>[8x]MHHHHHHTSLIEQPRWASKDSAAGAASTPDEKIVLEFMDALTSNDAAKLIEYFAEDTMYQNMPLPPAYGRDAVEQTLAGFFTVVSVDAVETFHIG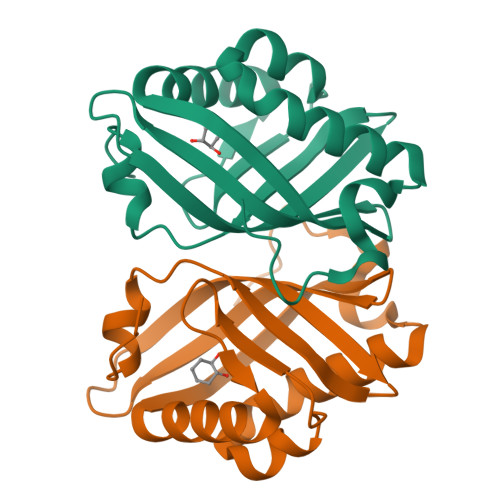SSNGLVYTERVDVLRALPTGKSYNFSILGVFQLTEGKITGWRDYFDLREFEEAVDLPLRG>[2x]GPLGSYGSRIEREQHHLIESIEKSTQYMAKRRIGALISVARDTGMDDYIETGIPLNAKISSQLLINIFIPNTPLHDGAVIIKGNEIASAASALPLSDSPFLSKELGTRHRAALGISEVTDSI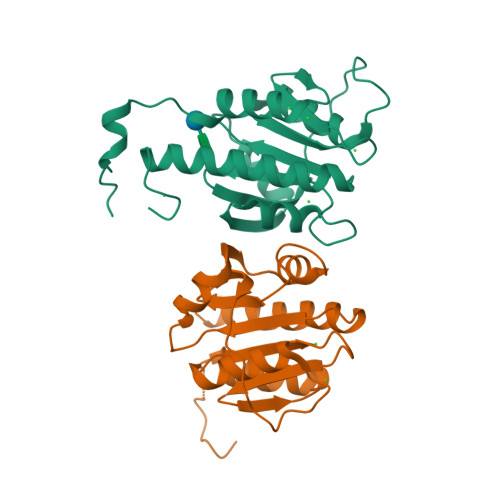TIVVSEETGGISLTKGGELFRDVSEEELHKILLKELVTVTAKKPSIFSKWKGGKSE> GPMSSVQLSRGDFHSIFTNKQRYDNPTGGVYQVYNTRKSDGANSNRKNLIMISDGIYHMKALLRNQAASKFQSMELQRGDIIRVIIAEPAIVRERKKYVLLVDDFELVQS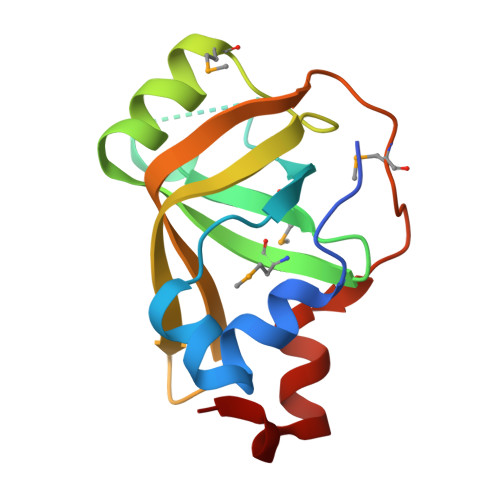RADMVNQTSTFLDNYFSEHPNETL> MSMSKQVLKENMKTTYHMDGSVNGHYFTIEGEGTGNPFKGQQSLKLRVTKGGPLPFAFDILSPTFTYGNRVFTDYPEYMPDYFKRSLPEGYSWERTMMYEDGATATASVRISLDKNGFVHKSTFHGENFPANGPVMKKKGVNWEP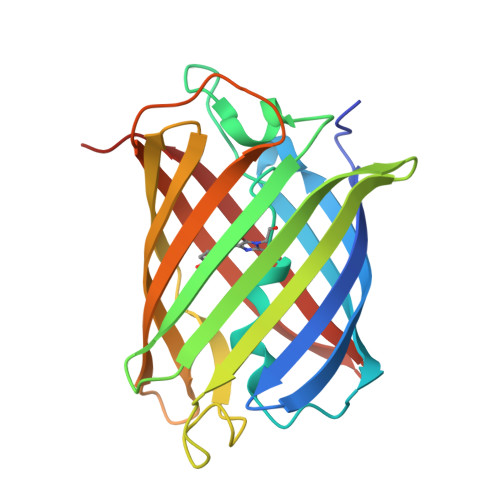SSETITPSDGILKGDVTMFLVLEGGQRLKALFQTTYKANKVVKMPPRHKIEHRLVRSEDGETIQLQEHAVAKYFTE> MQDNSRYTHFLTQHYDAKPQGRDDRYCESIMRRRGLTSPCKDINTFIHGNKRSIKAICENKNGNPHRENLRISKSSFQVTTCKLHGGSPWPPCQYRATAGFRNVVVACENGLP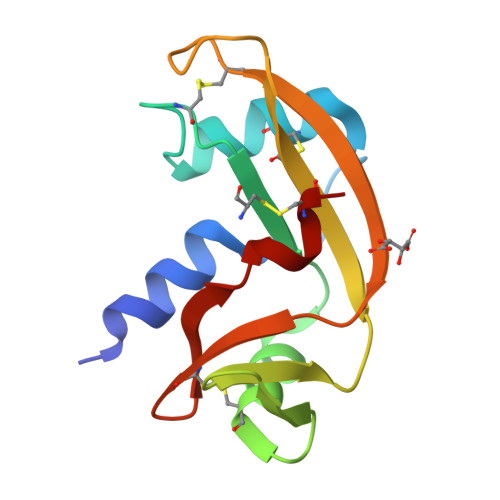VHLDQSIFCRP>[2x]SKELLAEYQDLTFLTKQEILLAHRRFCELLPQEQRSVESSLRAQVPFEQILSLPELKANPFKER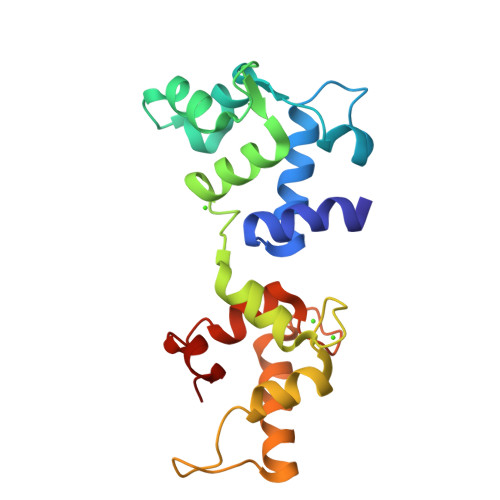ICRVFSTSPAKDSLSFEDFLDLLSVFSDTATPDIKSHYAFRIFDFDDDGTLNREDLSRLVNCLTGEGEDTRLSASEMKQLIDNILEESDIDRDGTINLSEFQHVISRSPDFASSFKIVL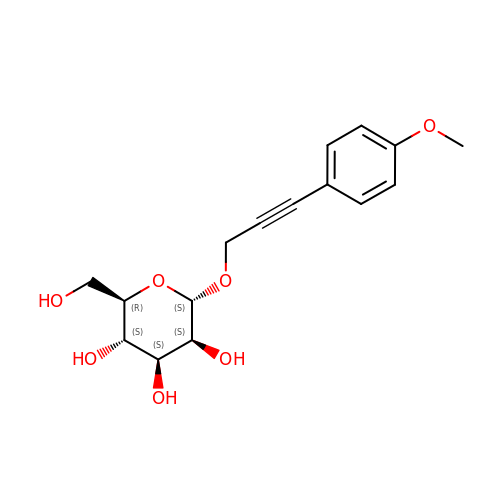3-(4-methoxyphenyl)prop-2-yn-1-yl alpha-D-mannopyranoside | C16 H20 O7 | UYJNIDIDTZJFNU-OWYFMNJBSA-N5-hydroxy-3-{1-[(2S)-2-hydroxy-3-{5-(methylsulfonyl)-3-[4-(trifluoromethyl)phenyl]-4,5,6,7-tetrahydro-1H-pyrazolo[4,3-c]pyridin-1-yl}propyl]piperidin-4-yl}-1H-pyrrolo[3,2-c]pyridin-5-ium | C29 H34 F3 N6 O4 S | 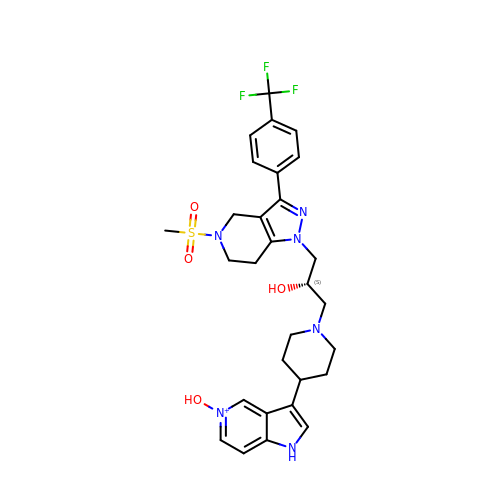OHGFFZPHDXPGML-QFIPXVFZSA-O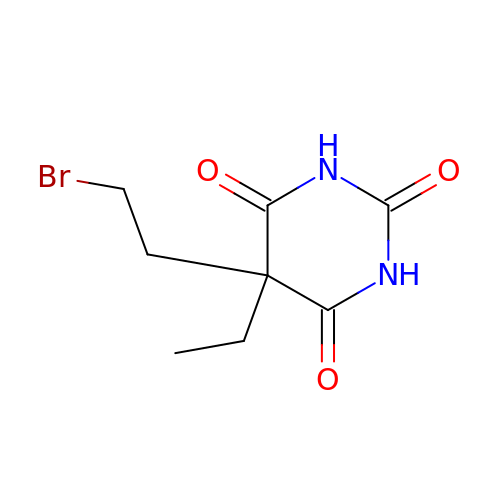5-(2-bromoethyl)-5-ethyl-1,3-diazinane-2,4,6-trione | C8 H11 Br N2 O3 | LJVTYPFTOBMROG-UHFFFAOYSA-N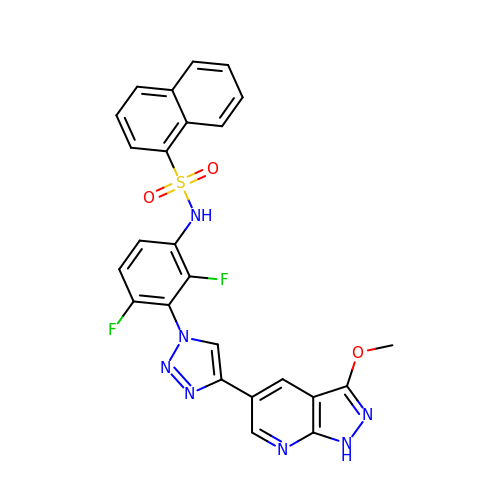~{N}-[2,4-bis(fluoranyl)-3-[4-(3-methoxy-1~{H}-pyrazolo[3,4-b]pyridin-5-yl)-1,2,3-triazol-1-yl]phenyl]naphthalene-1-sulfonamide | C25 H17 F2 N7 O3 S | RCRNSDSDZVDENT-UHFFFAOYSA-N octyl alpha-L-altropyranoside | C14 H28 O6 | 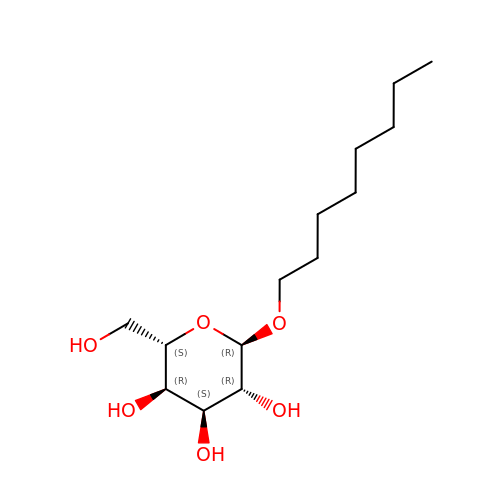HEGSGKPQLMEBJL-QSLWVIQJSA-N> GPLGSDFCGQWDTATAGDFTLYNDLWGESAGTGSQCTGVDSYSGDTIAWHTSWSWSGGSSSVKSYVNAALTFTPTQLNCISSIPTTWKWSYSGSSIVADVAYDTFLAETASGSSKYEIMVWLAALGGAGPISSTGSTIATPTIAGVNWKLYSGPNGDTTVYSFVADSTTESFSGDLNDFF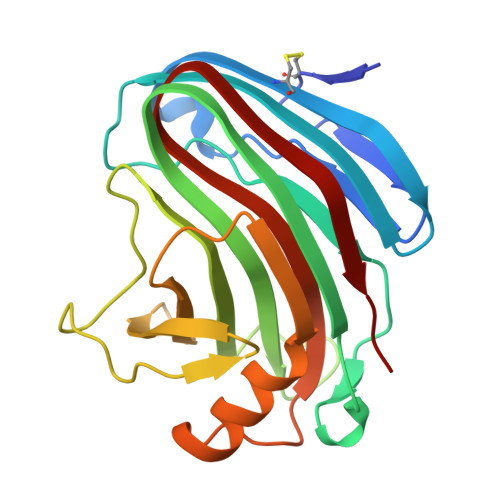TYLVDNEGVSDELYLTTLEAGTEPFTGSNAKLTVSEYSISIE>EPPLVFEPVTLESLRQEKGFQEVGKKQIKELDTLREKHAKERTSVQKTQNAAIDKLIKGKSKDDIRNDANIKNSINDQTKQWTDMIARHRKEEWDMLRQHVQDSQDAMKALMLTVQAAQIKQLEDRHARDIKDLNAKQAKMSADTAKEVQNDTLKTKNEKDRRLREKRQNNV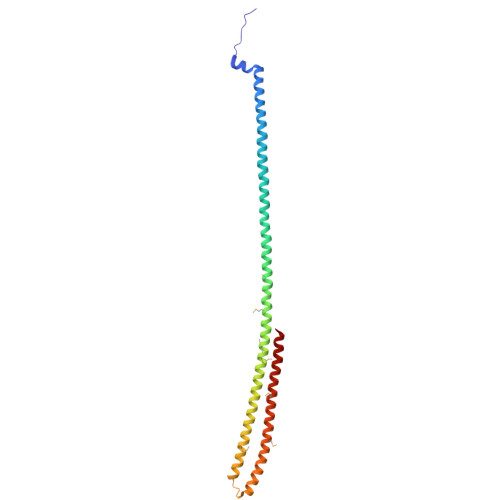KRFMEEKKQIGVKQGRAMEKLKLAHSKQIEEFSTDVQKL[2x]>STPKKNISKGAVLHEKPMTVMVLTATEPFNYKEGKENMFHATVATESKYYRVKVFNMDLKEKFTENQFITISKYFNSSGILEINETATVSEAAPNQMFEVPKNIIRSAKETLKISKIKELDSGTLIYGVFAVEKKKVNDKSITFKIKDNEDNIK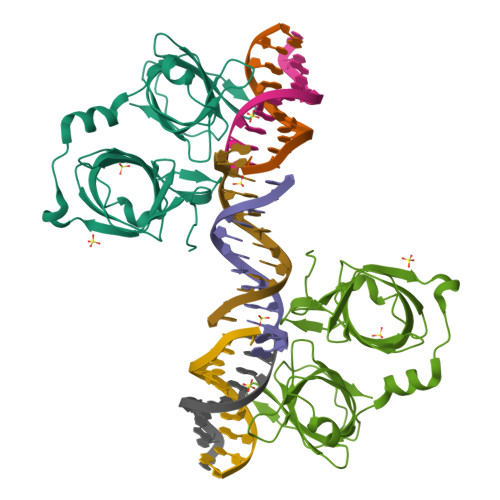VVWDKEQHNINYEKGDKLQLFSFHLRKGNGKPILHSGNHSFIKGE[2x]D-MYO-INOSITOL-1,4,5-TRIPHOSPHATE | C6 H15 O15 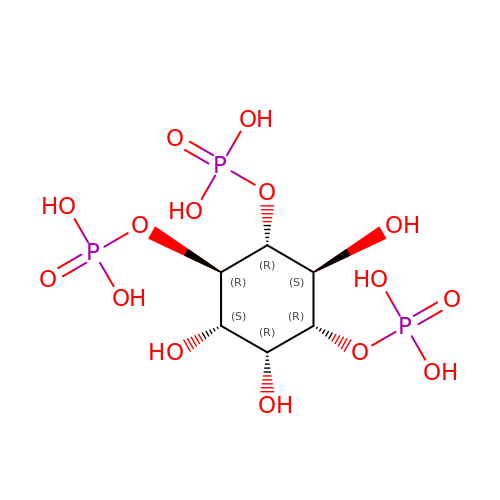P3 | MMWCIQZXVOZEGG-XJTPDSDZSA-N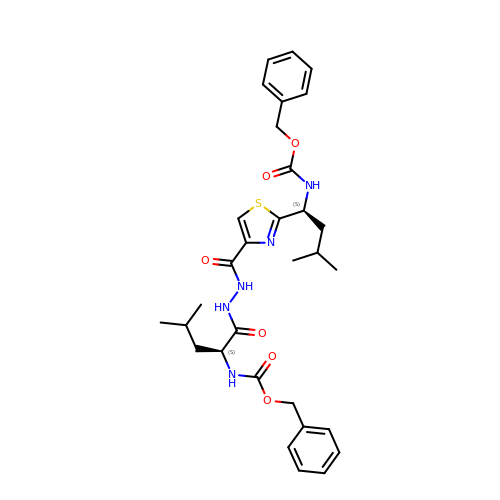N-[2-[1-(N-BENZYLOXYCARBONYLAMINO)-3-METHYLBUTYL]THIAZOL-4-YLCARBONYL]-N'-(BENZYLOXYCARBONYL-L-LEUCINYL)HYDRAZIDE | C31 H39 N5 O6 S | FNMSKYFYFLZDOO-DQEYMECFSA-N1-[2-(1H-indol-5-yloxy)ethyl]piperidine-4-carboxylic 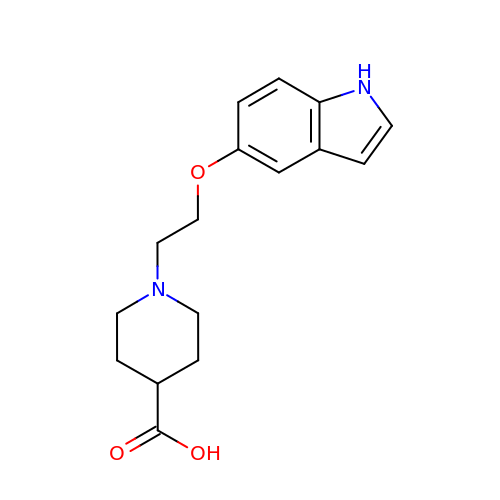acid | C16 H20 N2 O3 | WEUOMMCSMCVWHD-UHFFFAOYSA-N(2S,3S,4R,5R)-6-(HYDROXYAMINO)-2-(HYDROXYMETHYL)-2,3,4,5-TETRAHYDROPYRIDINE-3,4,5-TRIOL | C6 H12 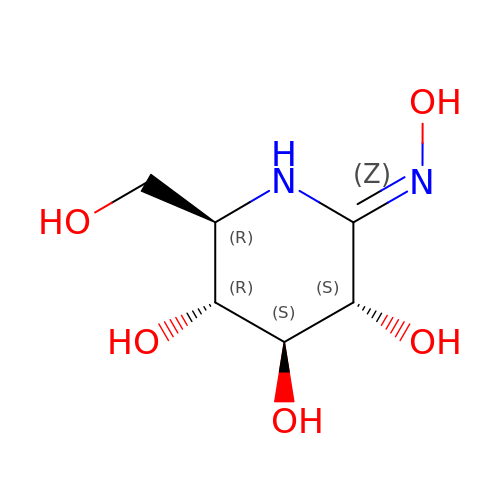N2 O5 | VBXHGXTYZGYTQG-SQOUGZDYSA-N>MGHHHHHHMDMTKIALLSDIHGNTTALEAVLADARQLGVDEYWLLGDILMPGTGRRRILDLLDQLPITARVLGNWEDSLWHGVRKELDSTRPSQRYLLRQCQYVLEEISLEEIEVLHNQPLQIHRQFGDLTVGISHHLPDKNWGRELIHTGKQEEFDRLVTHPPCDIAVYGHIHQQLLRYGTGGQLIVNPGSIGQPFFLDAQLRKDLRAQYMILEFDDKGLVDMDFRRVDYDVAAELQLAKDLRLPYFEVYYESLVNGIHHTHHQEFLRE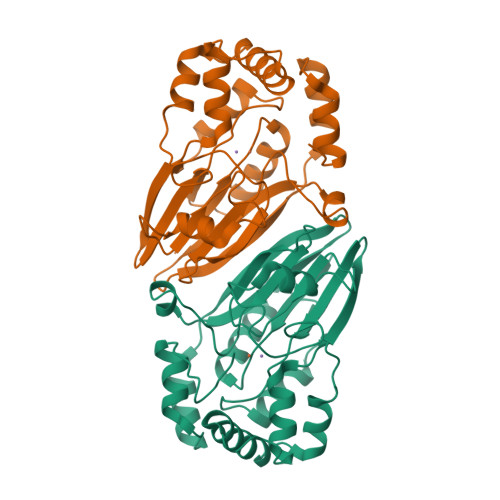[2x]>[6x]SMDDSETGFNLKVVLVSFKQCLDEKEEVLLDPYIASWKGLVRFLNSLGTIFSFISKDVVSKLRIMERLRGGPQSEHYRSLQAMVAHELSNRLVDLERRSHHPES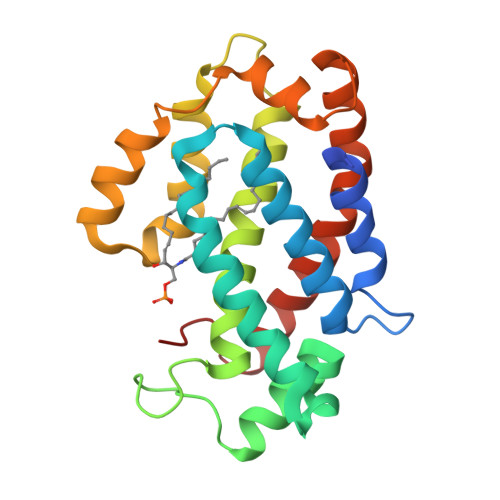GCRTVLRLHRALHWLQLFLEGLRTSPEDARTSALCADSYNASLAAYHPWVVRRAVTVAFCTLPTREVFLEAMNVGPPEQAVQMLGEALPFIQRVYNVSQKLYAEHSLLDLP>[2x]GSSEGYCSRILRAQGTRREGYTEFSLRVEGDPDFYKPGTSYRVTLSAAPPSYFRGFTLIALRENREGDKEEDHAGTFQIIDEEETQFMSNCPVAVTE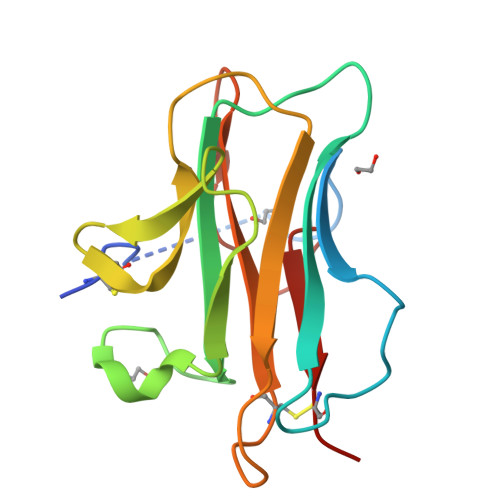STPRRRTRIQVFWIAPPAGTGCVILKASIVQKRIIYFQDEGSLTKKLCEQDS>[3x]PNPIPNFIHCRSYLDMLKVAVFRYLFWLVLVVVFVAGATRISIFGLGYLLACFYLLLFGTTLLQKDTRAQLVLWDCLILYNVTVIISKNMLSLLSCVFVEQMQSNFCWVIQLFSLVCTVKGYYDPKEMMTRDRDCLLPVEEAGIIWDSICFFFLLLQRRIFLSHYFLHVSADLKATALQASRGFALYNAANLKSINFHRQIEEKSLAQLKRQMKRIRAKQEKYRQSQASRGQLQSKDPQDPSQEPGPDSPGGSSPPRRQWWRPWLDHATVIHSGDYFLFESDSEEEEEALPEDPRPAAQSAFQMAYQAWVTNAQT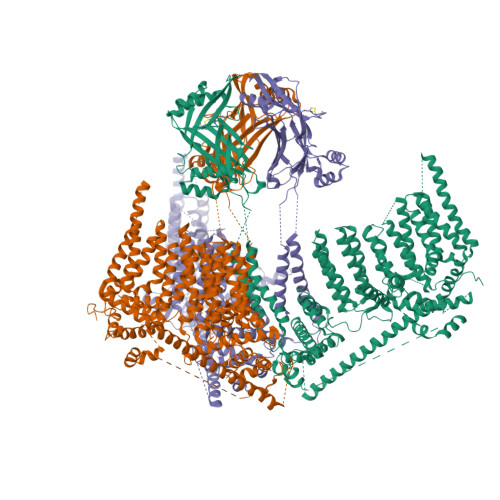VLRQRRERARQERAEQLASGGDLNPDVEPVDVPEDEMAGRSHMMQRVLSTMQFLWVLGQATVDGLTRWLRAFTKHHRTMSDVLCAERYLLTQELLRVGEVRRGVLDQLYVGEDEATLSGPVETRDGPSTASSGLGAEEPLSSMTDDXXXXXXXXXXXXXXXXXXXXXXXXXXXXXXXXXXXXXXXXXXXXXXXXXXXXXXXXXXXPELEEAERFEAQQGRTLRLLRAGYQCVAAHSELLCYFIIILNHMVTASAASLVLPVLVFLWAMLTIPRPSKRFWMTAIVFTEVMVVTKYLFQFGFFPWNSYVVLRRYENKPYFPPRILGLEKTDSYIKYDLVQLMALFFHRSQLLCYGLWDHEEDRYPKDHCRSSVKDREAKEEPEAKLESQSETGTGHPKEPVLAGTPRDHIQGKGSIRSKDVIQDPPEDLKPRHTRHISIRFRRRKETPGPKGTAVMETEHEEGEGKETTERKRPRHTQEKSKFRERMKAAGRRLQSFCVSLAQSFYQPLQRFFHDILHTKYRAATDVYALMFLADIVDIIIIIFGFWAFGKHSAATDIASSLSDDQVPQAFLFMLLVQFGTMVIDRALYLRKTVLGKLAFQVVLVVAIHIWMFFILPAVTERMFSQNAVAQLWYFVKCIYFALSAYQIRCGYPTRILGNFLTKKYNHLNLFLFQGFRLVPFLVELRAVMDWVWTDTTLSLSNWMCVEDIYANIFIIKCSRETEKKYPQPKGQKKKKIVKYGMGGLIILFLIAIIWFPLLFMSLIRSVVGVVNQPIDVTVTLKLGGYEPLFTMSAQQPSIVPFTPQAYEELSQQFDPYPLAMQFISQYSPEDIVTAQIEGSSGALWRISPPSRAQMKQELYNGTADITLRFTWNFQRDLAKGGTVEYTNEKHTLELAPNSTARRQLAQLLEGRPDQSVVIPHLFPKYIRAPNGPEANPVKQLQPDEEEDYLGVRIQLRREQVGTGASGEQAGTKASDFLEWWVIELQDCKADCNLLPMVIFSDKVSPPSLGFLAGYGIVGLYVSIVLVVGKFVRGFFSEISHSIMFEELPCVDRILKLCQDIFLVRETRELELEEELYAKLIFLYRSPETMIKWTREREKKLGAPLEVLFQ> SKTVHYLKDYQTPAYHILKTDLHFDINEPQTVVKSRLTVEPQRVGEPLVLDGSAKLLSVKINGAAADYVLEGETLTIAGVPSERFTVEVETEILPAENKSLMGLYASGGNLFTQCEPEGFRKITFYIDRPDVMSKFTTTIVADKKRYPVLLSNGN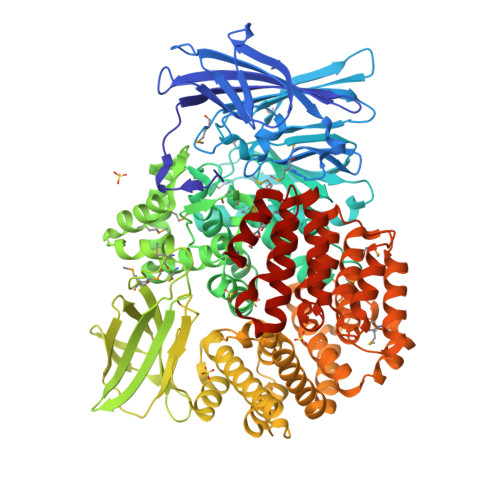KIDGGEFSDGRHWVKWEDPFSKPSYLFALVAGDLAVTEDYFTTMSGRNVKIEFYTTEADKPKVGFAVESLKNAMKWDETRFGLEYDLDIFMVVAVGDFNMGAMENKGLNIFNTKFVLADSRTATDTDFEGIESVVGHEYFHNWTGNRVTCRDWFQLSLKEGLTVFRDQEFSGDRASRAVRRIENIRLLRQHQFPEDAGPTAHPVRPASYEEMNNFYTMTVYEKGAEVVRMYHTLLGEEGFQKGMKLYFQRHDGQAVTCDDFRAAMADANGINLDQFALWYSQAGTPVLEAEGRLKNNIFELTVKQTVPPTPDMTDKQPMMIPVKVGLLNRNGEAVAFDYQGKRATEAVLLLTEAEQTFLLEGVTEAVVPSLLRGFSAPVHLNYPYSDDDLLLLLAHDSDAFTRWEAAQTLYRRAVAANLATLSDGVELPKHEKLLAAVEKVISDDLLDNAFKALLLGVPSEAELWDGAENIDPLRYHQAREALLDTLAVHFLPKWHELNRQAAKQENQSYEYSPEAAGWRTLRNVCRAFVLRADPAHIETVAEKYGEMAQNMTHEWGILSAVNGNESDTRNRLLAQFADKFSDDALVMDKYFALVGSSRRSDTLQQVRTALQHPKFSLENPNKARSLIGSFSRNVPHFHAEDGSGYRFIADKVIEIDRFNPQVAARLVQAFNLCNKLEPHRKNLVKQALQRIRAQEGLSKDVGEIVGKILD>[12x]GGACUCG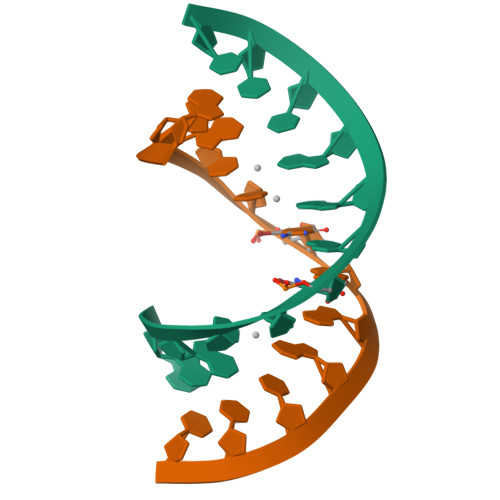AAUCC> ATTGTQGYTVVKNDWKKAVKQLQDGLKDNSIGKITVSFNDGVVGEVAPKSANKKADRDAAAEKLYNLVNTQLDKLGDGDYVDFSVDYNLENKIITNQADAEAIVTKLNSLNEKTLIDIATKDTFGMVSKTQDSEGKNVAATKALKVKDVATFGLKSGGSEDTGYVVEMKAGAVEDKYGKVGDSTAGIAINLPSTGLEYAGKGTTIDFNKTLKVDVTGGSTPSAVAVSGFVTKDDTDLAKSGTINVRVINAKEESIDIDAS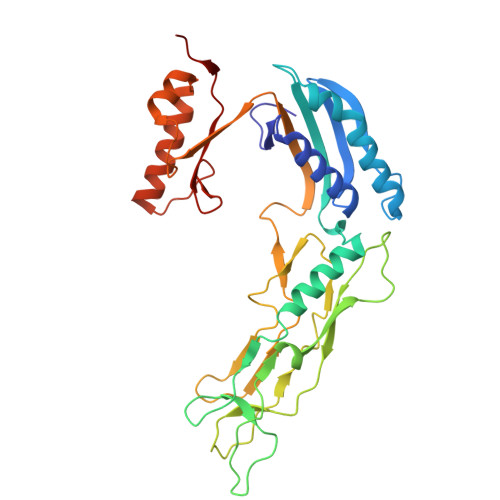SYTSAENLAKRYVFDPDEISEAYKAIVALQNDGIESNLVQLVNGKYQVIFYPEGKRLE(2S)-2-amino-3-methyl-1-(morpholin-4-yl)butan-1-one 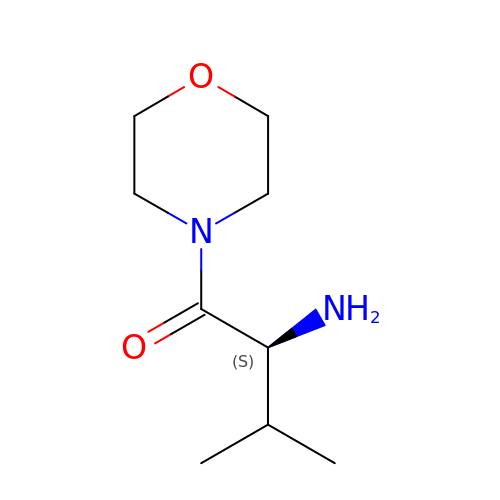| C9 H18 N2 O2 | GUDFDFVIXKMPIB-QMMMGPOBSA-N>MKPHPWFFGKIPRAKAEEMLSKQRHDGAFLIRESESAPGDFSLSVKFGNDVQHFKVLRDGAGKYFLWVVKFNSLNELVDYHRSTSVSRN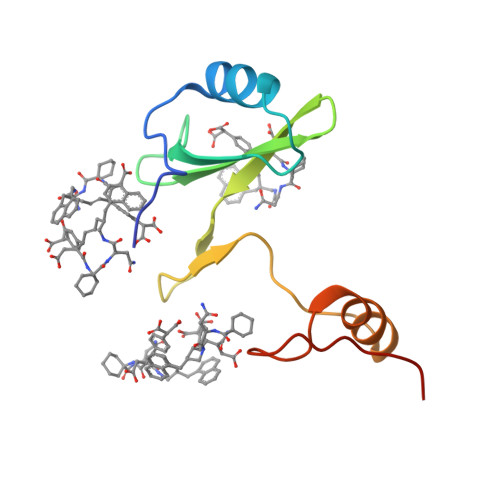QQIFLRDIEQ[4x]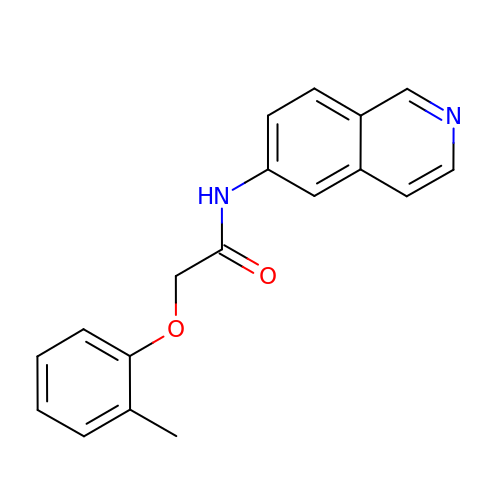~{N}-isoquinolin-6-yl-2-(2-methylphenoxy)ethanamide | C18 H16 N2 O2 | PEVCERQGPZRIFE-UHFFFAOYSA-N> GAMAPIITQSVEVDLPDATESQAVSSNDNPPVIVEVSGIGQYTVVVEKDRLERLPPEQVVAEVSSRFKANPKTVFLIGGAKDVPYDEIIKALNLLHSAGVKSVGLMTQPI

TolR is a 15-kDa inner membrane protein subunit of the Tol-Pal complex in Gram-negative bacteria, and its function is poorly understood. Tol-Pal is recruited to cell division sites where it is involved in maintaining the integrity of the outer membrane. TolR is related to MotB, the peptidoglycan (PG)-binding stator protein from the flagellum, suggesting it might serve a similar role in Tol-Pal. TolQ, TolR, and TolA are IM proteins that are coupled to the pmf through a conserved proton-conducting path, which is also found in MotA/MotB, ExbB/ExbD, and AglR/AglS.

Here, we present the 1.7-Å crystal structure of the intact periplasmic domain of E. coli TolR (TolR(36–142)). The final refined structure included residues 37–141, 161 solvent molecules, and 3 sodium ions. The monomer is composed of an N-terminal β-strand (β1 residues 41–47) and short α-helix (α1 residues 51–58) followed by a five-stranded mixed β-sheet (β2 residues 64–68; β3 residues 74–78; β4 residues 81–85; β5 residues 106–112, and β6 residues 133–139) sandwiched against two α-helices, α2 (residues 88–102) and α3 (residues 116–130). Close examination of TolR packing in the crystal revealed the presence of an intertwined dimer where the N-terminal β-strand of one subunit (β1) formed an anti-parallel β-sheet with the C terminus of a symmetry-related molecule (β6). The TolR(36–142) dimer interface is formed by residues from three regions as follows: the N terminus of the protein (residues 38–53 and 55), which includes β1 and part of α1; residues from the central regions of the protein that include β5 and α3 (residues 106, 108–118, 120–121, 124, and 127–128), and C-terminal β6 (residues 132–141). E. coli TolR(36–142) is also dimeric, but the architecture of the dimer is radically different from that of TolR(62–133) due to the intertwining of its N and C termini. TolR monomers are rotated ∼180° relative to each other as a result of this strand swapping, obliterating the putative PG-binding groove seen in TolR(62–133). In contrast, >2200 Å2 of accessible surface area is buried at the dimer interface of TolR(36–142), involving 44 residues from each monomer stabilized by 34 direct hydrogen bonds and 2 salt bridges. Truncated TolR (TolR(60–133)) bound PG but TolR(36–142) did not. Hence, this form of the stator protein likely represents the closed state of the pore, close to the membrane surface.>DEHNKNMADIEAAFEGRVGVYAINTGSGKAYSYRANERFPLCSSFKAFLAAAVLKMDQDSPGVLLEKVNYHNRTMEPHSPITEKFQSQGMAVGELAAATLQYSDNGAANLLMEKYIKGPEGMTQ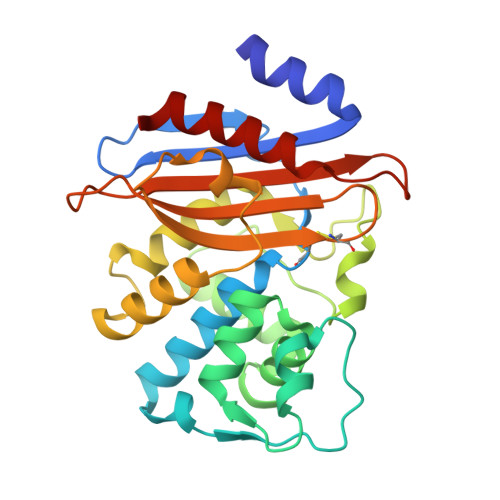FMNSIGDTKFRLDRWELDLNSAIPGDERDTSTPKAVAESLNKLISNTVLDNYHQEIFKKWMIGNTTGDNRIRAAVPDGWVVGDKTGTCGKYGTANDHAFILQGNNAAPLILSIYTTRKGEHMKHDDEVIAKAARIAIENVK[4x]>MAKNNAVAGFNALNGVELNLFTTDELKAIHYATMEVLMDPGIQVSDPEARQIFKENGCEVNEKTNVVKIPEYLVRKALQLAPSRFVLWGRDKKFNTVQECGGKVHWTCFGTGVKVCKYQDGKYVTVDSVEKDIADIAKLCDWAENIDYFSLPVSARDIAGQGAQDVHETLTPLANTAKHFHHIDPVGENVEYYRDIVKAYYGGDEEEARKKPIFSMLLCPTSPLELSVNACQVIIKGARFGIPVNVLSMAMSGGSSPVYLAGTLVTHNAEVLSGIVLAQLTVPGAK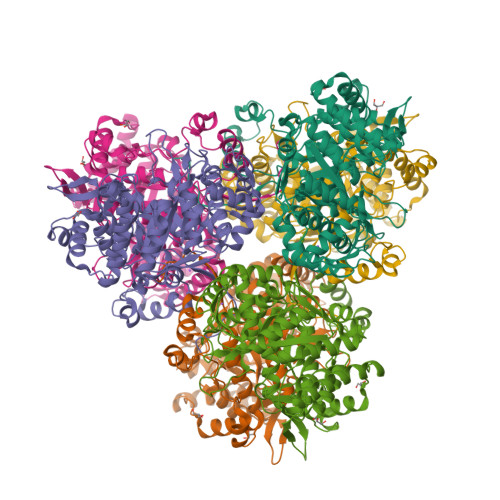VWYGSSTTTFDLKKGTAPVGSPELGLISAAVAKLAQFYGLPSYVAGSOSDAKVPDDQAGHEKTMTTLLPALAGANTIYGAGMLELGMTFSMEQLVIDNDIFSMVKKAMQGIPVSEETLAVESIQKVGIGNNFLALKQTRQLVDYPSNPMLLDRHMFGDWAAAGSKDLATVAHEKVEDVLKNHQVTPIDADIFKDMQAIVDKADKAFRGMGGHHHHHH[6x]> KPKLLNKFDKTIKAELDAAEKLRKRGKIEEAVNAFKELVRKYPQSPRARYGKAQCEDDLAEKRRSNEVLRGAIETYQEVASLPDVPADLLKLSLKRRSDRQQFLGHMRGSLLTLQRLVQLFPNDTSLKNDLGVGYLLIGDNDNAKKVYEEVLSVTPNDGFAKVHYGFILKAQNKIAESIPYL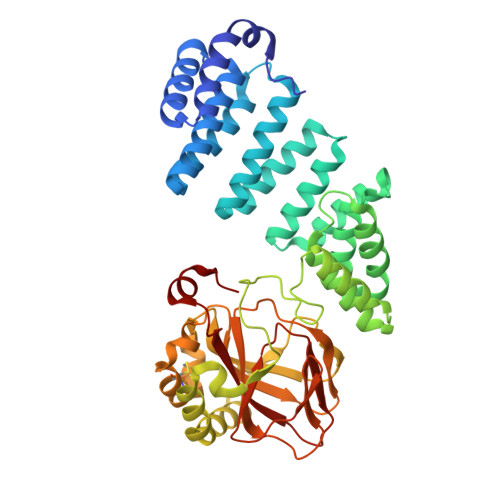KEGIESGDPGTDDGRFYFHLGDAMQRVGNKEAYKWYELGHKRGHFASVWQRSLYNVNGLKAQPWWTPKETGYTELVKSLERNWKLIRDEGLAVMDKAKGLFLPEDENLREKGDWSQFTLWQQGRRNENACKGAPKTCTLLEKFPETTGCRRGQIKYSIMHPGTHVWPHTGPTNCRLRMHLGLVIPKEGCKIRCANETKTWEEGKVLIFDDSFEAEVWQDASSFRLIFIVDVWHPELTPQQRRSLPAI>[2x]MAPERL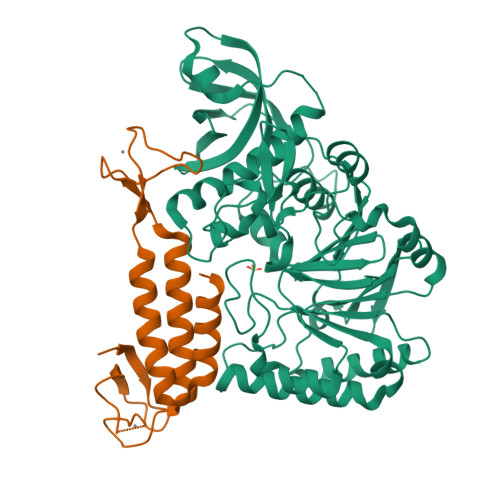RSRALSAFKLRGLLLRGEAIKYLTEALQSISELELEDKLEKIINAVEKQPLSSNMIERSVVEAAVQECSQSVDETIEHVFNIIGAFDIPRFVYNSERKKFLPLLMTNHPAPNLFGTPRDKAEMFRERYTILHQRTHRHELFTPPVIGSHPDESGSKFQLKTIETLLGSTTKIGDAIVLGMITQLKEGKFFLEDPTGTVQLDLSKAQFHSGLYTEACFVLAEGWFEDQVFHVNAFGFPPTEPSSTTRAYYGNINFFGGPSNTSVKTSAKLKQLEEENKDAMFVFLSDVWLDQVEVLEKLRIMFAGYSPAPPTCFILCGNFSSAPYGKNQVQALKDSLKTLADIICEYPDIHQSSRFVFVPGPEDPGFGSILPRPPLAESITNEFRQRVPFSVFTTNPCRIQYCTQEITVFREDLVNKMCRNCVRFPSSNLAIPNHFVKTILSQGHLTPLPLYVCPVYWAYDYALRVYPVPDLLVIADKYDPFTTTNTECLCINPGSFPRSGFSFKVFYPSNKTVEDSKLQGF;>[2x]AQFRDPCRSYVLPEVICRSCNFCRDLDLCKDSSFSEDGAVLPQWLCSNCQAPYDSSAIEMTLVEVLQKKLMAFTLQDLVCLKCRGVKETSMPVYCSCAGDFALTIHTQVFMEQIGIFRNIAQHYGMSYLLETLEWLLQKNPQLGH>[2x]GAMGMVSLVVPDLDVLRRWLDQQSITWFECDSCQALHLPHMQNFDGVFDAKIDLMDGVILFSALAEVKPTALIPLAGDLSQINASSLTVKAFLDIQDDNLPKLIVCQSLSAAAGLTYG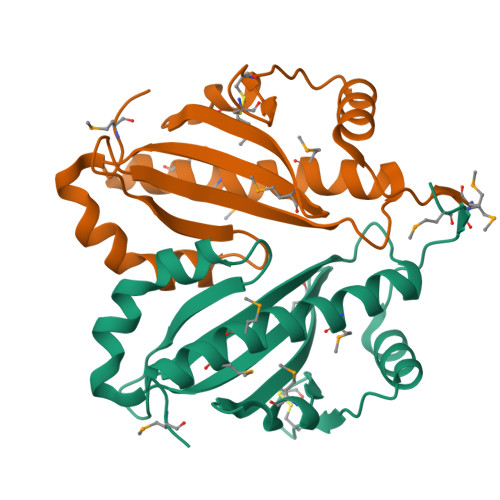QFVHFMKESEEQISMIVMEAFANHLLMIAEDEERPPMITSHSLLH> AIVIERPNVKWSDVAGLEGAKEALKEAVILPIKFPHLFTGKRTPWRGILLFGPPGTGKSYLAKAVATEANNSTFFSISSSDLVSKWLGESEKLVKNLFQLARENKPSIIFIDEIDSLCGSRSENESEAARRIKTEFLVQMQGVGVDNDGILVLGATNIPWVLDSAIRRRFEKRIYIPLPEPHARAAMFKLHLGTTQNSLTEADFRELGRKTDGYSGADISIIVRDALMQPVRKVQSATHFKKVRGPSRADPNHLVDDLLTPCSPGDPGAIEMTWMDVP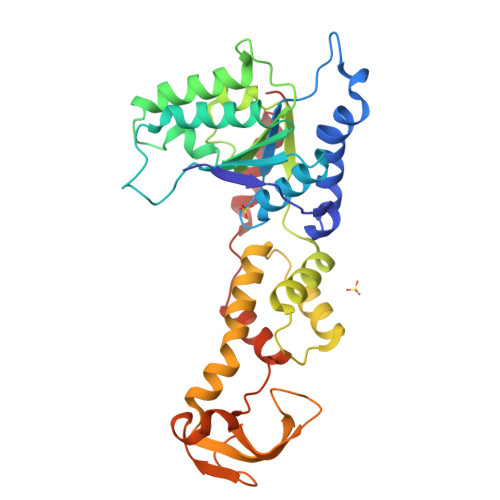GDKLLEPVVSMSDMLRSLSNTKPTVNEHDLLKLKKFTEDFGQEG>MFRLPTVMKQVRPVCRALAPHLTRAYAKDVKFGADARALMLQGVDLLADAVAVTMGPKGRTVIIEQSWGSPKVTKDGVTVAKSIDLKDKYKNIGAKLVQDVANNTNEEAGDGTTTATVLARAIAKEGFDTISKGANPVEIRRGVMMAVETVIKELKNLSKPVTTPEEIAQVATISANGDVEIGNIISNAMKKVGRKGVITVKDGKTLHDELEIIEGMKFDRGYISPYFINTAKGQKCEFQDAYLLLSEKKISSVQSIVPALEIANQHRKPLVIVAEDVDGEALSTLVLNRLKVGLQVVAVKAPGFGDNRKNQLRDMAVATGGTVFGDEAVGLALEDIQAHDFGKIGEVQITKDDTLLLKGGGSP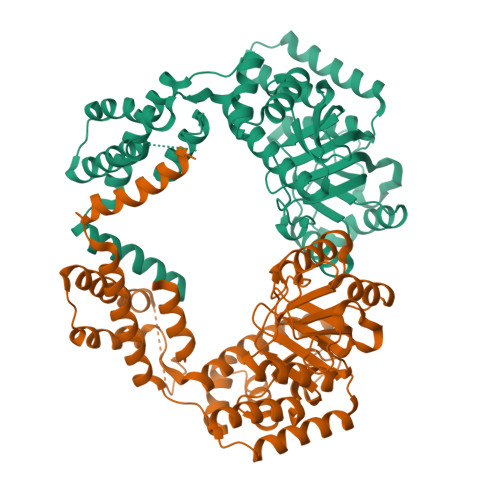AEVEKRAAEIVEQLENTTSDYEKEKLNERLAKLSDGVAVLKVGGTSDVEVNEKKDRVTDALNATRAAVEEGIVPGGGCALLRCIPSLDAIQTANADQKIGVEIIRRALRIPAMTIAKNAGVEGSLVVEKILQGSAELGYDAMQGEYVNMVEKGIIDPTKVVRTALLDAAGVASLLSTAEAVVTEIPKEEKEMPGGMGGMGGMGGMGGMGGGMGFLEHHHHHH[2x]N-[(2S)-3-azanyl-3-methyl-1-(oxidanylamino)-1-oxidanylidene-butan-2-yl]-4-[4-[(1R,2R)-2-(hydroxymethyl)cyclopropyl]buta-1,3-diynyl]benzamide 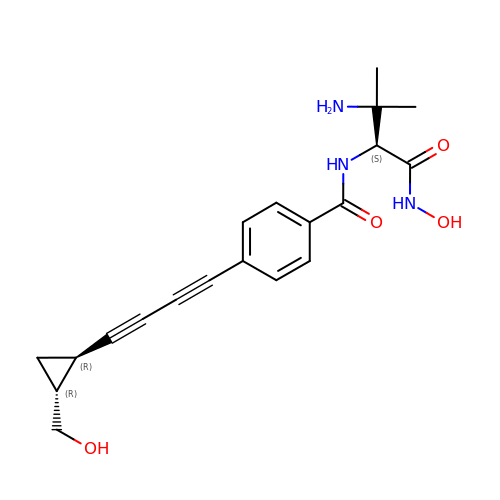| C20 H23 N3 O4 | GOCUUDXEOKIQRU-IXDOHACOSA-N> SNASQSLSVKTKKQWQKPDHKNPNPIAFILSSPRSGSTLLRVMLAGHPGLYSPPELHLLPFETMGDRHQELGLSHLGEGLQRALMDLENLTPEASQAKVNQWVKANTPIAD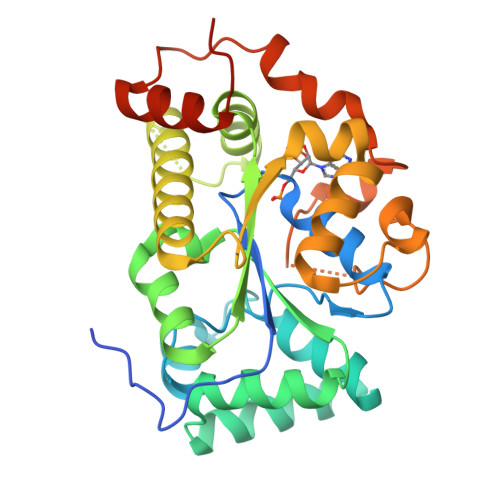IYAYLQRQAEQRLLIDKSPSYGSDRHILDHSEILFDQAKYIHLVRHPYAVIESFTRLRMDKLLGAEQQNPYALAESIWRTSNRNILDLGRTVGADRYLQVIYEDLVRDPRKVLTNICDFLGVDFDEALLNPYSGDRLTDGLHQQSMGVGDPNFLQHKTIDPALADKWRSITLPAALQLDTIQLAETFAYDLPQEPQLTPQTQ>[2x]MALTNAQILAVIDSWEETVGQFPVITHHVPLGGGLQGTLHCYEIPLAAPYGVGFAKNGPTRWQYKRTINQVVHRWGSHTVPFLLEPDNINGKTCTASQLCHNTRCHNPLHL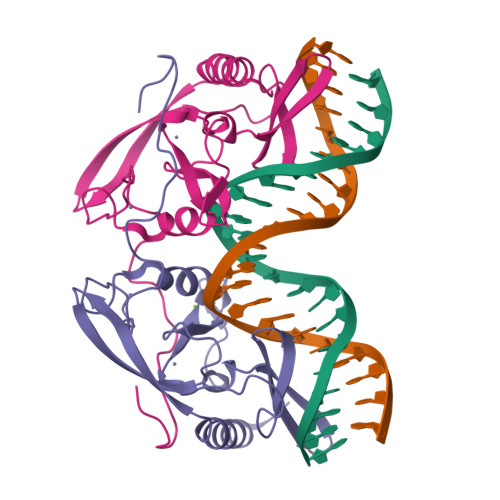CWESLDDNKGRNWCPGPNGGCVHAVVCLRQGPLYGPGATVAGPQQRGSHFVV>MGKYQVMKRA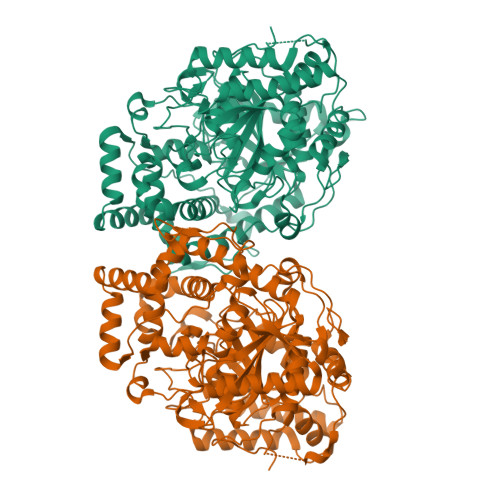SEVDLSTVKYKAETMKAPHLTGLSFKLFVNLLEAPLIGSLIVDYLKKDNGMTKIFRNTVIPEEPMFRPEFPSQEPEHDVVIVGEDESPIDRLETALKCLPQYDPSRSLHADPVSSFRYWKIRDYAYAYRSKLTTPLQVAKRIISIIEEFGYDKPPTPFLIRFDANEVIKQAEASTRRFEQGNPISVLDGIFVTIKDDIDCLPHPTNGGTTWLHEDRSVEKDSAVVSKLRSCGAILLGKANMHELGMGTTGNNSNYGTTRNPHDPKRYTGGSSSGSAAIVAAGLCSAALGTDGGGSVRIPSALCGITGLKTTYGRTDMTGSLCEGGTVEIIGPLASSLEDAFLVYAAILGSSSADRYNLKPSPPCFPKLLSHNGSNAIGSLRLGKYTKWFNDVSSSDISDKCEDILKLLSNNHGCKVVEIVVPELEEMRAAHVISIGSPTLSSLTPYCEAGKNSKLSYDTRTSFAIFRSFSASDYIAAQCLRRRLMEYHLNIFKDVDVIVTPTTGMTAPVIPPDALKNGETNIQVTTDLMRFVLAANLLGFPAISVPVGYDKEGLPIGLQIMGRPWAEATVLGLAAAVEELAPVTKKPAIFYDILNTNKGEFEAYVEQKLISEEDLNSAVDHHHHHH[2x]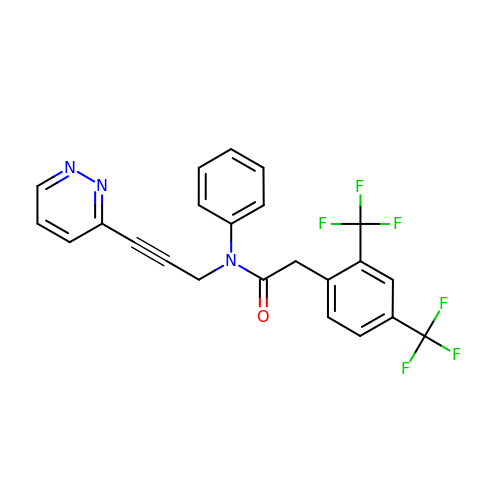2-[2,4-bis(trifluoromethyl)phenyl]-N-phenyl-N-[3-(pyridazin-3-yl)prop-2-yn-1-yl]acetamide | C23 H15 F6 N3 O | SCSRPWBBDHKGCX-UHFFFAOYSA-N> MGHHHHHH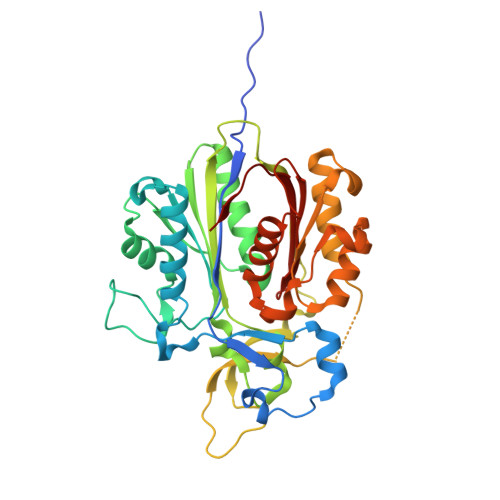AENLYFQGHMHKVKLAAITCELPARSYENDDPVFAAVPDLSESWWQFWGVNRRGYFDPRNGENEFSLVVRAAERLLRSSDTAPDSVDMLICSASSPIMTDAGDVLPDLRGRLYPRMANVLSKQLGLSRALPLDSQMECASFLLNLRLAASMIRQGKAEKVLVVCSEYISNLLDFTSRTSTLFADGCAVALLTRGDDDSCDLLASAEHSDATFYEVATGRWRLPENPTGEAKPRLYFSLFSDGQNKMASFVPTNVPIAMRRALEKAGLGSDDIDYFVFHQPAPFLVKAWAEGIGARPEQYQLTMGDTGVMISVSIPYTLMTGLREGKIRPGDRIVMAGAATGWGFAAQVWQLGEVLVC> KPFS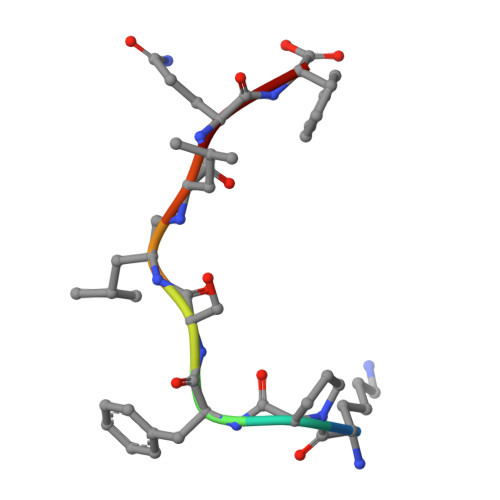XLQF> IEMKPHPWFFGKIPRAKAEEMLSKQRHDG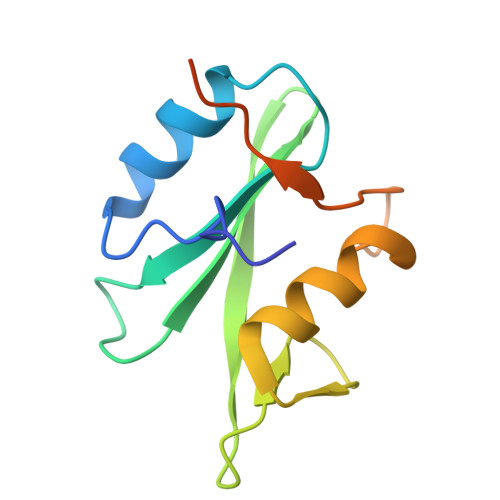AFLIRESESAPGDFSLSVKFGNDVQHFKVLRDGAGKYFLWVVKFNSLNELVDYHRSTSVSRNQQIFLRDIEQVPQQPTYVQAHHHHHH> MSKLDSLLKELPTRTAHLYRSIWHKYTEWLKTMPDLTGADLKLFLSQKYIVKYIASHDDIAKDPLPTCDAMIWFSRALDIENNDVLVLQQRLYGLVKLLEFDYSNVIAILQKISINLWNPSTDSLQSKHFKTCQDKLKLLLDFQWKFNTNVSFEDRTTVSLKDLQCILDDENGKCGLAHSSKPNFVLVPNFQSPFTCPIFTMAVYYYLRFHGVKKYYKGDGYQILSQLEHIPIIRGKSLDQYPRELTLGNWYPTIFKYCQLPYTKKHWFQVNQEWPQFPDFSDSSENTSTLAESDSENTIGIPDFYIEKMNRTKLQPCPQVHVHLFPTDLPPDIQAVFDLLNSVLVTSLPLLYRVFPTHDIFLDPSLKTPQNIAFLTGTLPLDIESQEHLL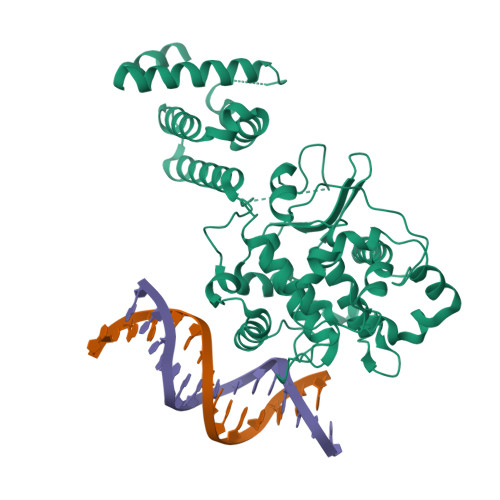AQLIDKTGTVSELVPNPVKIDQNEHTLTPIGTSLSQTDIPMLDQLKTELQKLIQLQTSTGFSQLITVLLEIFQRLDFKKSNKQFVIDLLQSCRKDMRNKLMDPCSLSTNFADELSDDENEKGNKTGAIYDPETDNGNEESVSD> GPGYQMADEIDAMALYRAWQQLDNGSCAQIRRVSEPDELRDIPAFYRLVQPFGWENPRHQQALLRMVFCLSAGKNVIRHQDKKSEQTTGISLGRALANS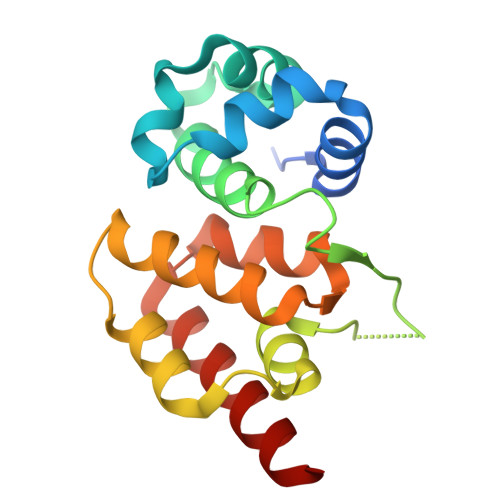GRINERRIFQLIRADRTADMVQLRRLLTHAEPVLDWPLMARMLTWWGKRERQQLLEDFVLTTNKNA> KLPST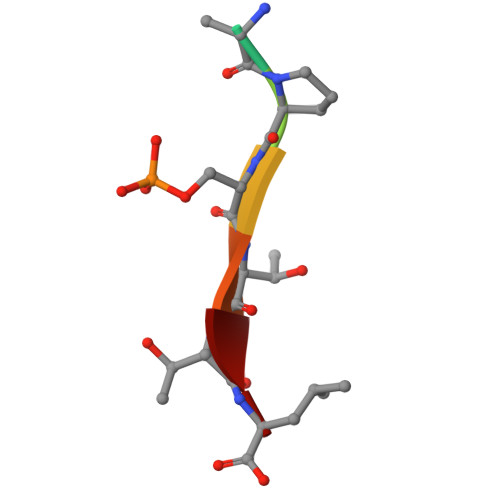TL> GGSNKSDLAALVSLVESVRHEQ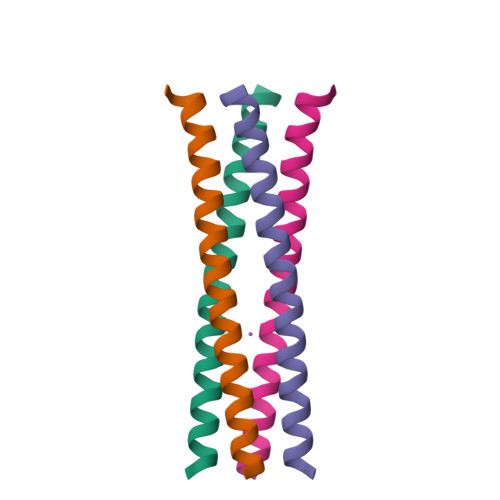QQLRNLCEMILEQQQRAKEFGENLYFQ>CGGREGVLKKLRAVENELHYNKSLLEEVKDELQKMRQ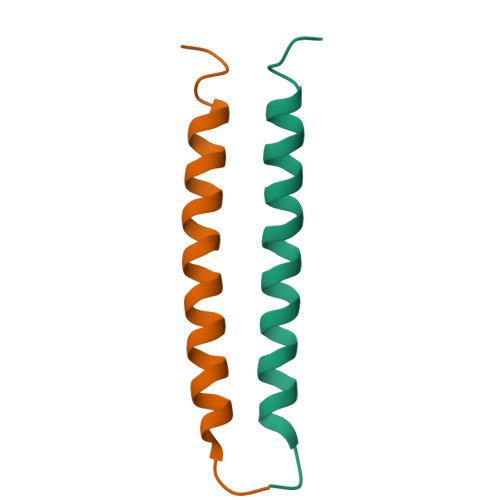L[2x]> DPSDRLVPELDTIVPLESTKAYNM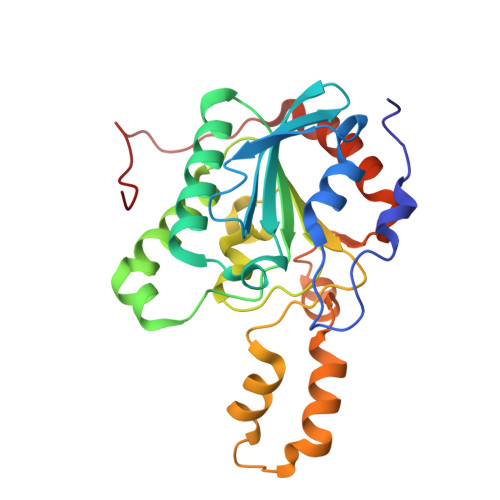VDIIHSVVDEREFFEIMPNYAKNIIVGFARMNGRTVGIVGNQPKVASGCLDINSSVKGARFVRFCDAFNIPLITFVDVPGFLPGTAQEYGGIIRHGAKLLYAFAEATVPKVTVITRKAYGGAYYVMSSKHLCGDTNYAWPTAEIAVMGAKGAVEIIFKGHENVEAAQAEYIEKFANPFPAAVRGFVDDIIQPSSTRARICCDLDVLASKKVQRPWRKHANIPL> GVRLASAFHQECSLQSCTQHQPYVVDDPCPIHFYSKWYIRVGARKSAPLIELCVDEAGSKSPIQYIDIGQYTVSCLPFTINCQEPKLGSLVVRCSFYEDF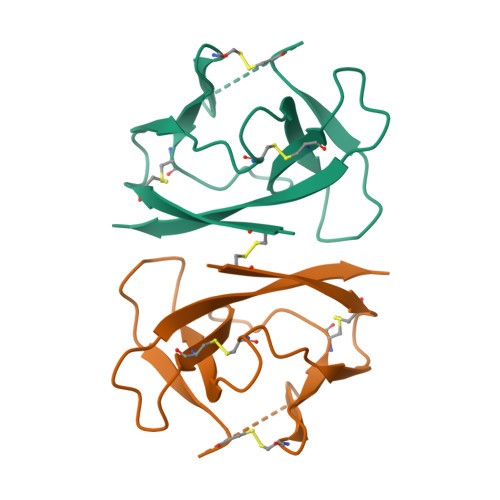LEYHDVRVVLDFI Olfactomedin-1 (Olfm1; also known as noelin and pancortin) is a member of the olfactomedin domain-containing superfamily and a highly expressed neuronal glycoprotein important for nervous system development. It binds a number of secreted proteins and cell surface-bound receptors to induce cell signaling processes. Using a combined approach of x-ray crystallography, solution scattering, analytical ultracentrifugation, and electron microscopy we determined that full-length Olfm1 forms disulfide-linked tetramers with a distinctive V-shaped architecture. The dimer-of-dimers architecture suggests a role for Olfm1 in clustering receptors to regulate signaling and sheds light on the conformation of several other olfactomedin domain family members.

Crystallization attempts of the full-length protein yielded no crystals, so we used limited proteolysis by α-chymotrypsin as a crystallization aid to remove unstructured regions. This yielded diffraction quality crystals and a data set to 2.4-Å resolution. The structure revealed a disulfide-linked dimer of β-propellers in the asymmetric unit related by a pseudo-2-fold rotation of 178°. In addition to the β-propellers, a segment of the coiled-coil domain (residues Val211–Leu225) was visible in the electron density. Cys221 in this coiled-coil segment forms an interprotein disulfide, covalently linking the two β-propellers. The dimer contacts are exclusively formed by the coiled coils; the two β-propellers are not contacting each other directly. Cys227, the first residue of the β-propeller, forms an intraprotein disulfide with Cys409 as predicted; this disulfide bond appears to close the β-propeller fold and lock it in a fixed orientation with respect to the coiled coil. Hence, the two β-propellers in the covalent dimer have a 60° angle between each other, resulting in an exposed outward orientation of the β-propeller top faces. The olfactomedin domain of Olfm1 forms a five-bladed β-propeller similar in structure to the recently solved olfactomedin domains of gliomedin, myocilin, and latrophilin3 (14–16). Remarkably, all glycosylation sites are located at either the side or the bottom of the β-propellers, whereas the top faces are free from glycans and completely exposed.

>MITNWMSQTLPSLVGLNTTRLSAASGGTLDRSTGVLPTNPEESWQVYSSAQDSEGRCICTVVAPQQTMCSRDARTKQLRQLLEKVQNMSQSIEVLDRRTQRDLQYVEKMENQMKGLETKFKQVEESHKQHLARQFKAIKAKMDELRPLIPVLEEYKADAKLVLQFKEEVQNLTSVLNELQEEIGAYDYDELQSRVSNLEERLRACMQKLACGKLTGISDPVTVKTSGSRFGSWMTDPLAPEGDNRVWYMDGYHNNRFVREYKSMVDFMNTDNFTSHRLPHPWSGTGQVVYNGSIYFNKFQSHIIIRFDLKTETILKTRSLDYAGYNNMYHYAWGGHSDIDLMVDENGLWAVYATNQNAGNIVISKLDPVSLQILQTWNTSYPKRSAGEAFIICGTLYVTNGYSGGTKVHYAYQTNASTYEYIDIPFQNKYSHISMLDYNPKDRALYAWNNGHQTLYNVTLFHAAAHHHHHH[2x]> MKPVKVKTPAG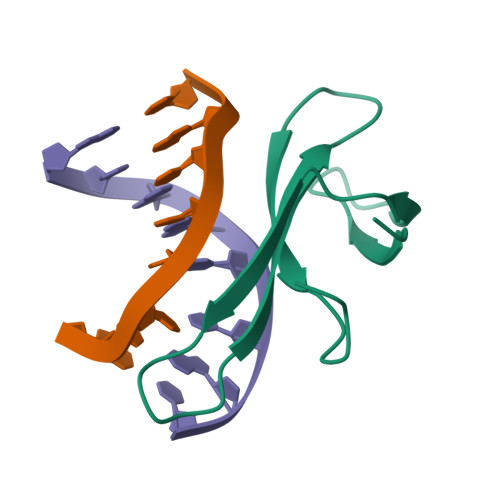KEAELVPEKVWALAPKGRKGVKIGLFKDPETGKYFRHKLPDDYPI> EKEEAIFRSAEMALVQFYIPQEISRDSAYTLGQLGLVQFRDLNSKVRAFQRTFVNEIRRLDNVERQYRYFYSLLKKHDIKLYEGDTDKYLDGSGELYVPPSGSVIDDYVRNASYLEERLIQMEDATDQIEVQKNDLEQYRFILQSGDEFFLKGDNTDSTSYMDEDMIDANGENIAAAIGASVNYVTGVIARDKVATLEQILWRVLRGNLFFKTVEIEQPVYDVKTREYKHKNAFIVFSHGDLIIKRIRKIAESLDANLYDVDSSNEGRSQQLAKVNKNLSDLYTVLKTTSTTLESELYAIAKELDSWFQDVTREKAIFEILNKSNYDTNRKILIAEGWIPRDELATLQARLGEMIARLGIDVPSIIQVLDTNHTPPTFHRTNKFTAGFQSICDCYGIAQYREINAGLPTIVTFPFMFAIMFGDMGHGFLMTLAALSLVLNEKKINKMKRGEIFDMAFTGRYIILLMGVFSMYTGFLYNDIFSKTMTIFKSGWKWPDHWKKGESITATSVGTYPIGLDWAWHGTENALLFSNSYKMKLSILMGFIHMTYSYFFSLANHLYFNSMIDIIGNFIPGLLFMQGIFGYLSVCIVYKWAVDWVKDGKPAPGLLNMLINMFLSPGTIDDELYPHQAKVQVFLLLMALVCIPWLLLVKPLHFKFTHKKKSHEPLPSTEADASSEDLEAQQLISAMDADDAEEEEVGSGSHGEDFGDIMIHQVIHTIEFCLNCVSHTASYLRLWALSLAHAQLSSVLWTMTIQIAFGFRGFVGVFMTVALFAMWFALTCAVLVLMEGTSAMLHSLRLHWVESMSKFFVGEGLPYEPFAFEYKDM;> MEGVYFNIDNGFIEGVVRGYRNGLLSNNQYINLTQCDTLEDLKLQLSSTDYGNFLSSVSSESLTTSLIQEYASSKLYHEFNYIRDQSSGSTRKFMDYITYGYMIDNVALMITGTIHDRDKGEILQRCHPLGWFDTLPTLSVATDLESLYETVLVDTPLAPYFKNCFDTAEELDDMNIEIIRNKLYKAYLEDFYNFVTEEIPEPAKECMQTLLGFEADRRSINIALNSLQSSDIDPDLKSDLLPNIGKLYPLATFHLAQAQDFEGVRAALANVYEYRGFLETGNLEDHFYQLEMELCRDAFTQQFAISTVWAWMKSKEQEVRNITWIAECIAQNQRERINNYISVY;> SFSHFLYYLVLIVVIVYGLYKLFTGHGSDINFGKFLLRTSPYMWANLGIALCVGLSVVGAAWGIFITGSSMIGAGVRAPRITTKNLISIIFCEVVAIYGLIIAIVFSSKLTVATAENMYSKSNLYTGYSLFWAGITVGASNLICGIAVGITGATAAISDAADSALFVKILVIEIFGSILGLLGLIVGLLMAGKASEFQ;> SNIYAPLYAPFFGFAGCAAAMVLSCLGAAIGTAKSGIGIAGIGTFKPELIMKSLIPVVMSGILAIYGLVVAVLIAGNLSPTEDYTLFNGFMHLSCGLCVGFACLSSGYAIGMVGDVGVRKYMHQPRLFVGIVLILIFSEVLGLYGMIVALILNTRGSE;>MTELCPVYAPFFGAIGCASAIIFTSLGAAYGTAKSGVGICATCVLRPDLLFKNIVPVIMAGIIAIYGLVVSVLVCYSLGQKQALYTGFIQLGAGLSVGLSGLAAGFAIGIVGDAGVRGSSQQPRLFVGMILILIFAEVLGLYGLIVALLLNSRATQDVV[8x];> MSSFYTVVGVFIVVSAMSVLFWIMAPKNNQAVWRSTVILTLAMMFLMWAITFLCQLHPLVAPRRSDLRPEF;> DDILSSIWTEGLLMCLIVSALLLFILIVALSWISNLDITYGALEKSTNPIKK;> TGKAWCCTVLSAFGVVILSVIAHLFNTNHESFVGSINDPEDGPA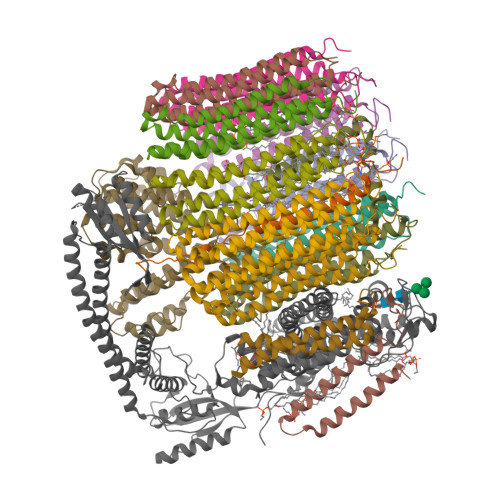VAHTVYLAALVYLVFFVFCGFQVYL>MTTFLIKHKASGKFLHPYGGSSNPANNTKLVLHSDIHERMYFQFDVVDERWGYIKHVASGKIVHPYGGQANPPNETNMVLHQDRHDRALFAMD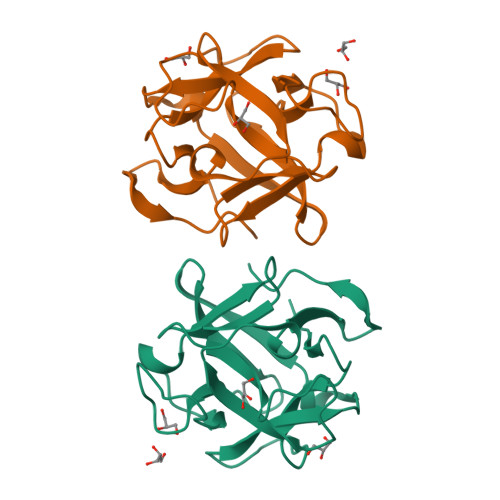FFNDNIMHKGGKYIHPKGGSPNPPNNTETVIHGDKHAAMEFIFVSPKNKDKRVLVYAHHHHHH[2x]> DNGAGEETKSYAETYRLTADDVANINALNESAPAASSAGPSFRAPDSDDRVTPPAEPLDRMPDPYRPSYGRAETVVNNY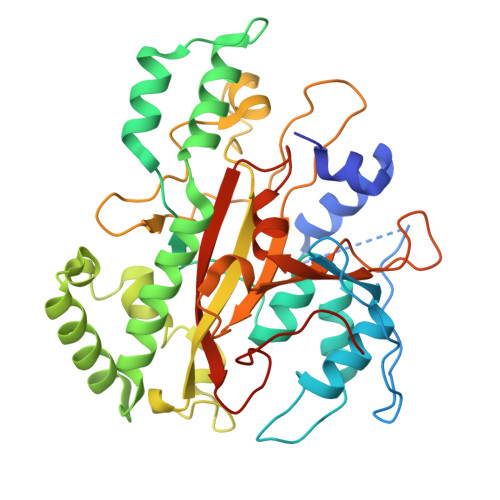IRKWQQVYSHRDGRKQQMTEEQREWLSYGCVGVTWVNSGQYPTNRLAFASFDEDRFKNELKNGRPRSGETRAEFEGRVAKESFDEEKGFQRAREVASVMNRALENAHDESAYLDNLKKELANGNDALRNEDARSPFYSALRNTPSFKERNGGNHDPSRMKAVIYSKHFWSGQDRSSSADKRKYGDPDAFRPAPGTGLVDMSRDRNIPRSPTSPGEGFVNFDYGWFGAQTEADADKTVWTHGNHYHAPNGSLGAMHVYESKFRNWSEGYSDFDRGAYVITFIPKSWNTAPDKVKQGWPHHHHHH> MATDVAQGPNGRALAESMNPDLLSAIQQHISIERYASVTYLAMSIWCAERELAGFYQFFDGAAKDEQSHAVHFTQYLIARSQSNDLQTLDAPRQNWDSLASLMATAFQMEADTTSSIQSVYALAERNSDTRTTVFLDPLIEAQIQSEDQFAYLLGRVKFANGDPTALLVIDNELRAG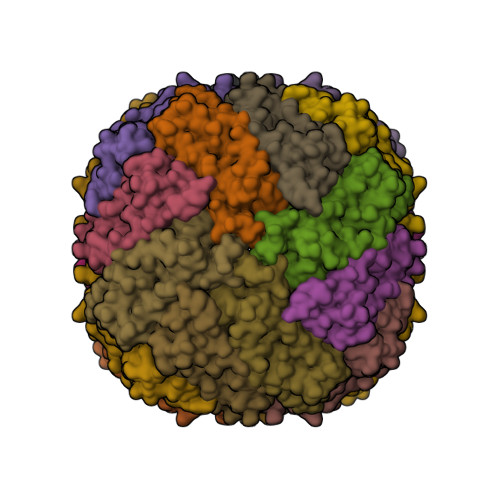QTQRG>GHHHHHHVPAFLSKLWTLVEETHTNEFITWSQNGQSFLVLDEQRFAKEILPKYFKHNNMASFVRQLNMYGFRKVVHIDSGIVKQERDGPVEFQHPYFKQGQDDLLENIKRKVS[3x]

Heat shock factor 1 (HSF1) and 2 (HSF2) play distinct but overlapping regulatory roles in maintaining cellular proteostasis or mediating cell differentiation and development. Upon activation, both HSFs trimerize and bind to heat shock elements (HSEs) present in the promoter region of target genes. HSFs recognize and bind HSEs through the DBD, which is the most conserved and only structurally characterized domain. Here, we present co-crystal structures of human HSF1 and HSF2 trimers bound to DNA, which reveal a triangular arrangement of the three DNA-binding domains (DBDs) with protein-protein interactions largely mediated by the wing domain.

HSF2-DBD was crystallized in complex with a canonical three-site HSE, 21 bp with a 5′-overhang. The structure refined at 1.75 Å reveals an HSF2 trimer bound to the three nGAAn repeats in unambiguous electron density. The DNA in the crystal was packed in a head-to-tail manner, where the 5′-overhung adenine in one strand formed a standard Watson-Crick base pair with the 5′-overhung thymine in the complementary strand from a neighboring asymmetric unit. In this structure, an HSF2 trimer binds to a tripartite HSE motif with one-to-one occupancy between the DBDs and the nGAAn repeats. All DBDs sit on one-half of DNA and are spatially arranged like an equilateral triangle seen from the top. Noticeably, the C-terminal peptide of each DBD stretches toward the triangle center across the DNA axis and obviously positions the downstream coiled coil at an approximate 3-fold symmetry axis, which relates the three DBDs within a single trimer. Exceptionally, the side chain of Arg109 close to the C terminus in DBD II deeply inserts into the major groove and engages in a direct hydrogen bond with the purine preceding TTC. This arginine in the other two DBDs, however, contacts two neighboring nucleobases by bifurcated solvent-mediated hydrogen bonds (S4C and, S4D). Likewise, the wing domain in HSF2 DBD I, albeit not entirely visible in electron density, is engaged in a similar hydrogen bond network with DBD III. In the HSF2 trimer-binding structure, however, obvious bending is observed at the 5′-proximal TTC triplet bound by DBD I rather than the downstream purine-pyrimidine base pair, while the DNA at the other two binding sites remains a relatively linear shape.>[3x]SNAYKNYFPKEPERIVYDKERVLQPIHNQLKGINIENVKIKEKEVVNATVDELQKMIDDGKLSYEELTSIYLFRIQEHDQNGIT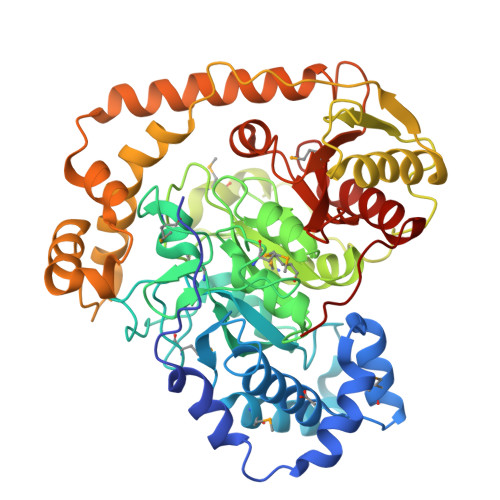LNSVTEINPNAMEEARKLDQERSRNKKSNLYGIPVVVKDNVQTAKVMPTSAGTYVLKDWIADQDATIVKQLKEEGAFVLGKANMSEWANYLSFTMPSGYSGKKGQNLNPYGPIMFDTSGSSSGSATVVAADFAPLAVGTETTGSIVAPAAQQSVVGLRPSLGRVSRTGIIPLAETLDTAGPMARTVKDAATLFNAMIGYDEKDVMTEKVKDKERIDYTKDLSIDGLKGKKIGLLFSVDQQDENRKAVAEKIRKDLQDAGAILTDYIQLNNGGVDNLQTLEYEFKHNVNDYFSQQKNVPVKSLKEIIAFNKRDSNRRIKYGQTLIEASEKSTITKDEFEKVVQTSQENAKKELNKYLVEKGLDALVMINNEEVLLSAVAGYPELAVPAGYDNNGEPVGAVFVGKQFGEKELFNIGYAYEQQSKNRKPPKL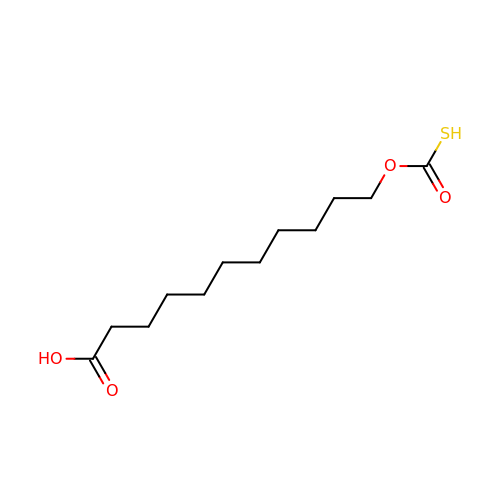11-[(MERCAPTOCARBONYL)OXY]UNDECANOIC ACID | C12 H22 O4 S | XSZQJZYGKSSUAF-UHFFFAOYSA-N> MEKEITELTKIRREFPNKKFSSTDMKKAGKLLKAEGPDAVRDFLNSCQEIIGDFKPPVKTNIVSISRPFEEWPVSMVGRAIQEYYFSLTKEELESVHPGTSSEDHKSFFNITGLSNYNYTSVQGLNLIFKNAKAIYDGTLVKANNKNKKLEKKFNEINHKRSLEGLPIITPDFEEPFDENGHLNNPPGINRNIYGYQGCAAKVFVPSKHKMVSLPKEYEGYNRDPNLSLAGFRNRLEIPEGEPGHVPWFQRMDIPEGQIGHVNKIQRFNFVHGKNSGKVKFSDKTGRVKRYHHSKYKDATKPYKFLEESKKVSALDSILAIITIGDDWVVFDIRGLYRNVFYRELAQKGLTAVQLLDLFTGDPVIDPKKGVVTFSYKEGVVPVFSQKIVPRFKSRDTLEKLTSQGPVALLSVDLGQNEPVAARVCSLKNINDKITLDNSCRISFLDDYKKQIKDYRDSLDELEIKIRLEAINSLETNQQVEIRDLDVFSADRAKANTVDMFDIDPNLISWDSMSDARVSTQISDLYLKNGGDESRVYFEINNKRIKRSDYNISQLVRPKLSDSTRKNLNDSIWKLKRTSEEYLKLSKRKLELSRAVVNYTIRQSKLLSGINDIVIILED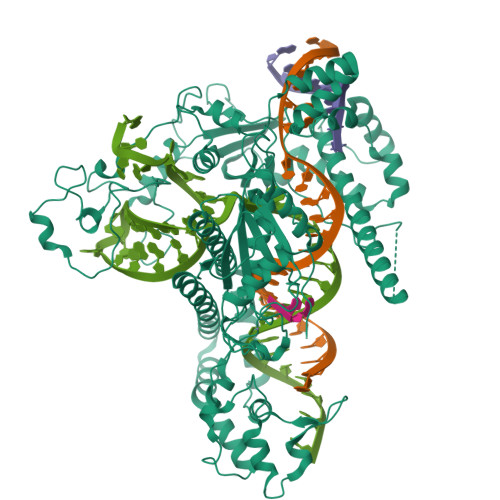LDVKKKFNGRGIRDIGWDNFFSSRKENRWFIPAFHKAFSELSSNRGLCVIEVNPAWTSATCPDCGFCSKENRDGINFTCRKCGVSYHADIDVATLNIARVAVLGKPMSGPADRERLGDTKKPRVARSRKTMKRKDISNSTVEAMVTA> GSHMSLSKQVVPTHRVEIAPNSESTAKMDHSNYQHNGLITKIWGTAGWTFNHAVTFGYPLNPTSDDKRRYKNYFISLGDVLPCRLCRESYKKFITTGKTALTNEVLRNRHTLTKWFYDVHNAVNNKLEVDYGLSYEDVVNKYESFRAKCGKPVPTVKGCVTPLDHKAFSFKKLYYMDAPIVSLDKVENFVRIARMRGISDKYFAFLELATVLNGDFNELKKQSSWEYRNKYAQKKIRHMRENAIPSIEEQGYWKGTPTIDELKLLLFLASNLNRTEVNDAINNVERLESTHYIEN

Mimivirus R596 is an enzyme of the Erv family of sulfhydryl oxidases, which catalyze the formation of disulfide bonds using an active-site di-cysteine motif juxtaposed to a flavin adenine dinucleotide (FAD) cofactor. Erv disulfide catalysts are apparently universal in eukaryotic species and are a highly conserved element of NCLDVs as well. Here we present the structure of the intact mimivirus sulfhydryl oxidase R596, including both its sulfhydryl oxidase domain and its ORFan domain. The mimivirus R596 enzyme contains an additional domain not found in other sulfhydryl oxidases from either cells or viruses, and this domain does not share detectable sequence homology with any other known protein.

Mimivirus R596-4C was crystallized in space group P6122 with one protomer in the asymmetric unit. Diffraction data were collected to 2.21 Å resolution. The R596-4C structure is highly helical and has a two-domain architecture. Rather than clustering spatially with the carboxy-terminal helices of R596, helix α6 packs against helix α5 from its own chain and helix α1 from the Erv domain of the other protomer (α1’). The tightly intertwined R596-4C dimer has a larger buried surface area (1150 Å2) than the R596Erv dimer alone (680 Å2). The R596-4C ORFan domain (R596-4CORFan, residues 180–292) is composed of six helices, α7 through α12. A structure similarity search found no close match for R596-4CORFan, suggesting that it represents a new fold. In contrast, residues 229 and 266, which are cysteines in wild-type R596 but alanines in R596-4C, are buried in the R596-4CORFan core and likely form a disulfide bond in the wild-type protein. In the R596-4C structure, these cysteines, Cys146 and Cys156, appear to be within 10 Å of the FAD-proximal cysteine pair, Cys 80 and Cys83, from the symmetry-related subunit (left). Notably, the lack of clear electron density seen for Cys146, Cys156, and the intervening loop in the R596-4C crystal structure (right) implies that the loop may be sufficiently mobile to approach the FAD-proximal cysteines.>SNKISCLPRVAQNLGYHYSPDLPGFCPIPKELAEHWPVVSNDRYPNCLQITLQQVCELSKPCSAGYMVGQSVFVQTPGVTSYWLTEWVDGKARALPDSLFSSGRFETNSRAFLDEAEEKFAAAHPHACLGEINKSTVGGSHFIFSQYLPPLLPADAVALVGASLAGKAAAA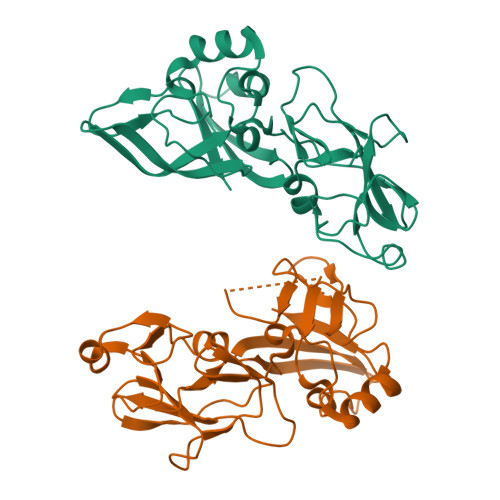ACSVVDVYAPSFEPYLHPETLSRVYKIMIDFKPCRLMVWRNATFYVQE[6x]> MVKKNDLFVDVSSHNGYDITGILEQMGTTNTI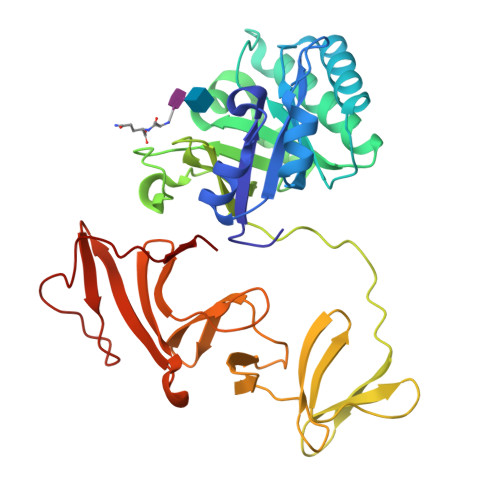IKISESTTYLNPCLSAQVEQSNPIGFYHFARFGGDVAEAEREAQFFLDNVPMQVKYLVLDYQDDPSGDAQANTNACLRFMQMIADAGYKPIYYSYKPFTHDNVDYQQILAQFPNSLWIAGYGLNDGTANFEYFPSMDGIRWWQYSSNPFDKNIVLLDDEEDDKPKTAGTWKQDSKGWWFRRNNGSFPYNKWEKIGGVWYYFDSKGYCLTSEWLKDNEKWYYLKDNGAMATGWVLVGSEWYYMDDSGAMVTGWVKYKNNWYYMTNERGNMVSNEFIKSGKGWYFMNTNGELADNPSFTKEPDGLITVA> MMEYEDLELITIWPSPTKNKLCQFIKQNLSKEHVVTQLFFIDATSSFPLSQFQKL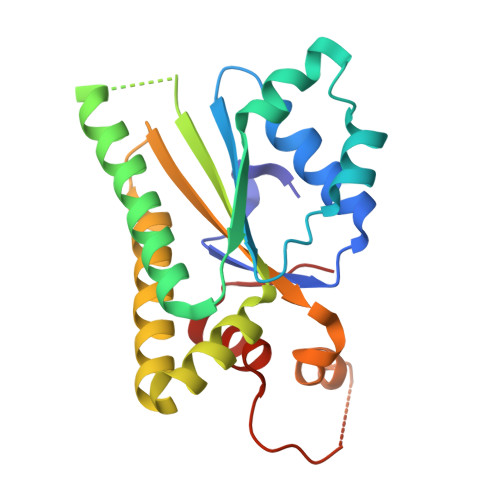VPPTLPENVRIYENIRINTCLDLEELSAITVKLLQILSMNKINAQRGTEDAVTEPLKIILYINGLEVMFRNSQFKSSPQRSHELLRDTLLKLRVMGNDENENASIRTLLEFPKEQLLDYYLKKNNNTRTSSVRSKRRRIKNGDSLAEYIWKYYADSLFE>[16x]VLPENMKRYMGRDAQRMNILAGRIIAETVRSTLGPKGMDKMLVDDLGDVVVTNDGVTILREMSVEHPAAKMLIEVAKTQEKEVGDGTTTAVVVAGELLRKAEELLDQNVHPTIVVKGYQAAAQKAQELLKTIACEVGAQDKEILTKIAMTSITGKGAEKAKEKLAEIIVEAVSAVVDDEGKVDKDLIKIEKKSGASIDDTELIKGVLVDK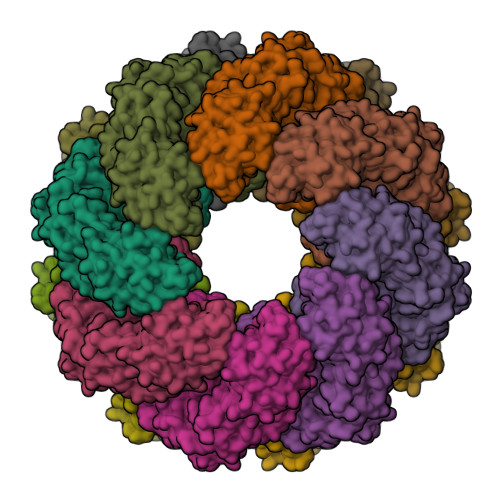ERVSAQMPKKVTDAKIALLNCAIEETASEMLKDMVAEIKASGANVLFCQKGIDDLAQHYLAKEGIVAARRVKKSDMEKLAKATGANVIAAIAALSAQDLGDAGLVEERKISGDSMIFVEECKHPKAVTMLIRGTTEHVIEEVARAVDDAVGVVGCTIEDGRIVSGGGSTEVELSMKLREYAEGISGREQLAVRAFADALEVIPRTLAENAGLDAIEILVKVRAAHASNGNKCAGLNVFTGAVEDMCENGVVEPLRVKTQAIQSAAESTEMLLRIDDVIAAE> MEQ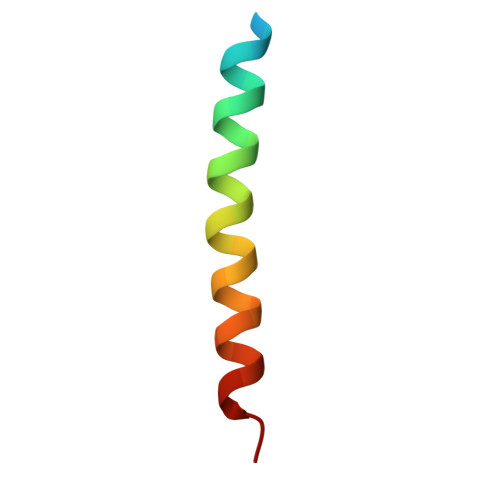VADFDTIYQAMIQISVVLCFALGIIAGGQR>MNSNLPAENLTIAVNMTKTLPTAVTHGFNSTNDPPSMSITRLFPALLECFGIVLCGAIAGRANVITSTQAKGLGNFVSRFALPALLFKNMVVLNFSNVDWSFLYSILIAKASVFFIVCVLTLLVASPDSRFSKAGLFPIFATQSNDFALGYPIVEALYQTTYPEYLQYIYLVAPISLMMLNPIGFIFCEIQKWKDTQNASQNKIKIVGLGLLRVLQNPIVFMVFIGIAFNFILDRKVPVYVENFLDGLGNSFSGSALFYLGLTMVGKIKRLKKSAFVVLILLITAKLLVLPLLCREMVELLDKGDSVVNHTSLSNYAFLYGVFPVAPGVAIFATQFNMEVEIITSGMVISTFVSAPIMYVSAWLLTFPTMDPKPLAYAIQNVSFDISIVSLISLIWSLAILLLSKKYKQLPHMLTTNLLIAQSIVCAGMMIWNFVKEKNFVGQILVFVLLYSSLYSTYLWTGLLAISLFLLKKRERVQIPVGIIIISGWGIPALLVGVLLITGKHNGDSIDSAFFYGKEQMITTAVTLFCSILIAGISLMCMNQTAQAGSYEGFDQSQSHKVVEPGNTAFEESPAPVNEPELFTSSIPETSCCSCSMGNGELHCPSIEPIANTSTSEPVIPSFEKNNHCVSRCNSQSCILAQEEEQYLQSGDQQLTRHVLLCLLLIIGLFANLSSCLWWLFNQEPGRLYVELQFFCAVFNFGQGFISFGIFGLDKHLIILPFKRRLEFLWNNKDTAENRDSPVSEEIKMTCQQFIHYHRDLCIRNIVKERRCGAKTSAGT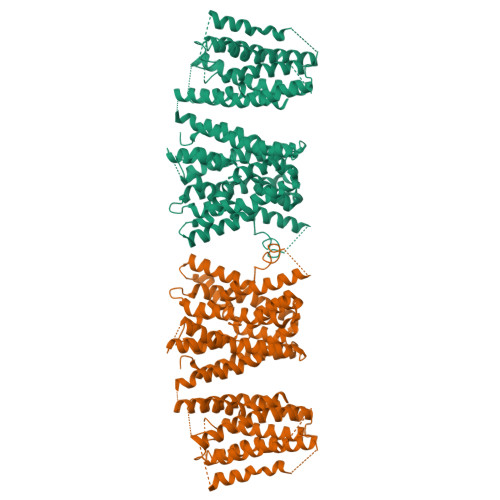FCGCDLVSWLIEVGLASDRGEAVIYGDRLVQGGVIQHITNEYEFRDEYLFYRFLQKSPEQSPPAINANTLQQERYKEIEHSSPPSHSPKTSRENLYFQ[2x]>[2x]MAQTVPYGIPLIKADKVQAQGFKGANVKVAVLDTGIQASHPDLNVVGGASFVAGEAYNTDGNGHGTHVAGTVAALDNTTGVLGVAPSVSLYAVKVLNSSGSGSYSGIVSGIEWATTNGMDVINMSLGGASGSTAMKQAVDNAYARGVVVVAAAGNSGNSGSTNTIGYPAKYDSVIAVGAVDSNSNRASFSSVGAELEVMAPGAGVYSTYPTNTYATLNGTSMASPHVAGAAALIL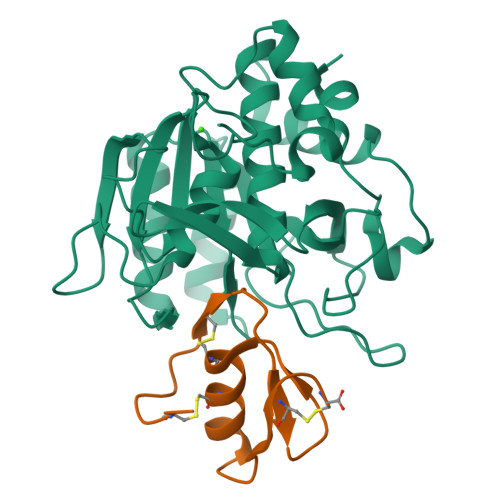SKHPNLSASQVRNRLSSTATYLGSSFYYGKGLINVEAAAQ;>[2x]VEVDCSRFPNTTNEEGKDVLVCTEDLRPICGTDGVTHSECLLCAYNIEYGTNISKEHDGECREAVPMDCSRYPNTTSEEGKVMILCNKALNPVCGTDGVTYDNECVLCAHNLEQGTSVGKKHDGECRKELAAVSVDCSEYPKPACTLEYRPLCGSDNKTYGNKCNFCNAVVESNGTLTLSHFGKC>[2x]KTVIKNETGTISISQLNKNVWVHTELGSFNGEAVPSNGLVLNTSKGLVLVDSSWDDKLTKELIEMVEKKFQKRV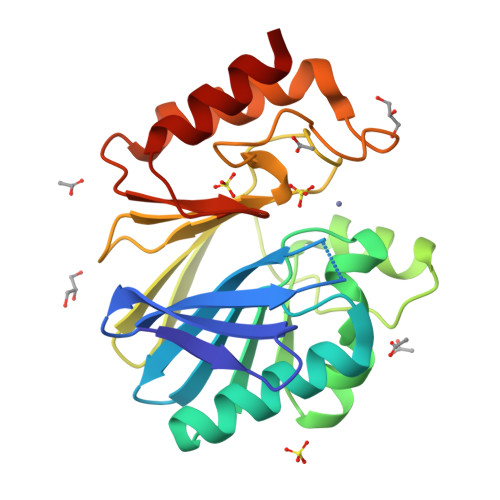TDVIITHAHADHIGGIKTLKERGIKAHSTALTAELAKKNGYEEPLGDLQTVTNLKFGNMKVETFYPGKGHTEDNIVVWLPQYNILVGGSLVKSTSAKDLGNVADAYVNEWSTSIENVLKRYRNINAVVPGHGEVGDKGLLLHTLDLLK>GMDYQEYQQFLARINTARDACVAKDIDVDLLMARHDYFGRELCKSLNIEYRNDVPFIDIILDIRPEVDPLTIDAPHITPDNYLYINNVLYIIDYKVSVSNESS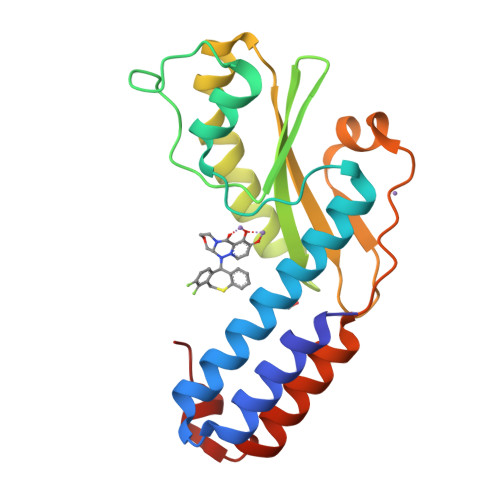VITYDKYYELTRDISDRLSIPIEIVIIRIDPVSRDLHINSDRFKELYPTIVVDINFNQFFDLKQLLYEKFGDDEEFLLKVA[4x]> SGIVPTLQNIVATVTLGCRLDLKTVALHARNAEYNPKRFAAVIMRIREPKTTALIFASGKMVVTGAKSEDDSKLASRKYARIIQKIGFAAKFTDFKIQNIVGSCDVKFPIRLEGLAFSHGTFSSYEPELFPGLIYRMVKPKIVLLIFVSGKIVLTGAKQREEIYQAFEAIYPVLSEFRKM;> SNAEASRVYEIIVESVVNEVREDFENAGIDEQTLQDLKNIWQKKLTETKVTTF;> GSSALLDTDEVGSELDDSDDDYLISEGEEDGPDENLMLCLYDKVTRTKARWKCSLKDGVVTINRNDYTFQKAQVEAEWV;> AVPGYYELYRRSTIGNSLVDALDTLISDGRIEASLAMRVLETFDKVVAETLKDNTQSKLTVKGNLDTYGFCDDVWTFIVKNCQ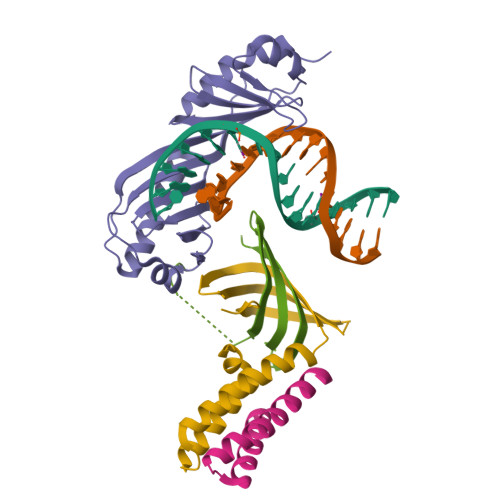VTVEDSHRDASQNGSGDSQSVISVDKLRIVACNSKKSE> GSHMVATVKRTIRIKTQQHILPEVPPVENFPVRQWSIEIVLLDDEGKEIPATIFDKVIYHLHPTFANPNRTFTDPPFRIEEQGWGGFPLDISVFLLEKAGERKIPHDLNFLQESYEVEH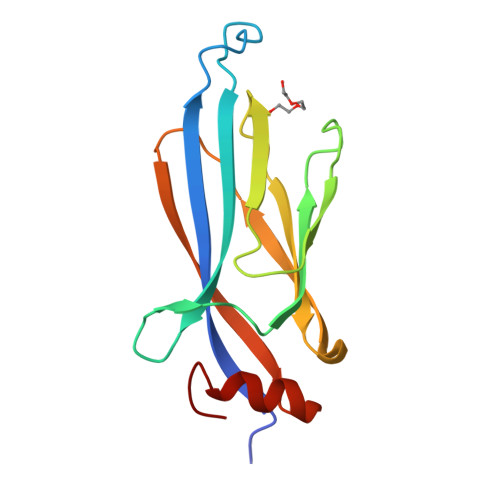VIQIPLNKPLLTEELAKSGST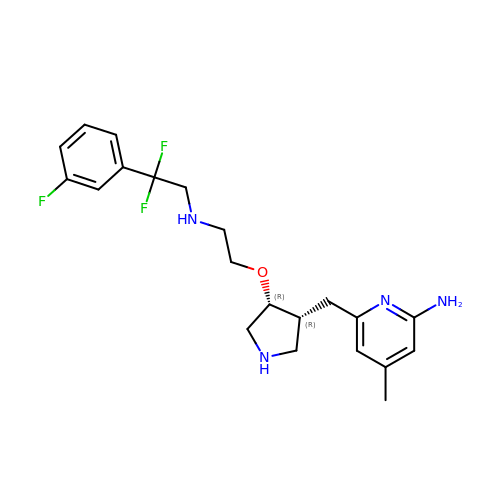6-{[(3R,4R)-4-(2-{[2,2-difluoro-2-(3-fluorophenyl)ethyl]amino}ethoxy)pyrrolidin-3-yl]methyl}-4-methylpyridin-2-amine | C21 H27 F3 N4 O | IRAITVAESBBILD-BEFAXECRSA-N Tripartite α-PFTs are members of the ClyA α-PFT family. Proteins in this family undergo a large scale conformational change from a compact soluble structure, where the hydrophobic residues are hidden often within a β-tongue motif, to an extended pore structure with the hydrophobic residues exposed in two extended α-helices which insert into the cell membrane. Here we show that S. marcescens has a tripartite haemolytic α-PFT (SmhABC), and propose a mechanism of pore assembly. We present the structures of the soluble A component (SmhA), as well as the soluble and pore conformations of the B component (SmhB).

To further investigate the differences in lytic activity between SmhABC and AhlABC the crystal structure of soluble SmhA was determined to 2.78 Å in space group P212121. This crystal form contained four closely related molecules in the asymmetric unit (rmsD Cα between molecules of 0.4–0.6 Å), with no oligomeric structures observed. SmhA folds into two distinct domains, a compact five helical bundle (α1, α2, α3, α6 and α7), and an associated head domain containing two helices (α4 and α5), and the β-tongue domain (two long anti-parallel β-strands, β1 and β2). In all monomers, there is missing density for approximately 20 residues between β1 and β2 (G208 – A229). Residues E192-V205 (β1 and loop to α3) and Y231-N250 (β2 and loop to α4) of the β-tongue domain are largely hydrophobic containing only polar uncharged and nonpolar residues, and are buried in the core of the protein, packing against α1, α3, α4, α5 (residues A272-Q283), and residues N351-E367 at the C-terminus. However, in SmhA, NheA and Hbl-B, this region has an additional extended loop and short helix that extends the length of the tail domain, a feature not observed in SmhB or AhlB. AhlB and SmhB use both a short β-strand and a short helix connected by a loop, while SmhA uses only a short loop perpendicular to β1. As soluble SmhA, SmhB and AhlB all share very similar structures, we propose that the head domain of SmhA would also unfold into its pore form about 2 hinges in the same way as seen in SmhB and AhlB, with hinge 1 between α3 and α4, and α5 and α6, and hinge 2 between α4 and β1, and α5 and β2. This would result in the pore form of SmhA having a similar extended helical structure to that of AhlB and SmhB. In this model the mixed hydrophobic/hydrophilic residues of the β-tongue head of SmhA form two extended amphipathic helices 36 Å in length at the ends of α3 and α4,, sufficient to cross the membrane, and thus with the potential to form a hydrophilic lining to the pore.

>[4x]MNNLTSIDLSPQTLMAMHISISSQALLNQSYSNLLLSQQLLTSQSMDPGLTVKIKAYQNQLRQQAQVFKQNTVAELIGLYTKASNFAALVNAVNALYSTEDPQVSQKGAEMVAALSDVAQHYQAAAQAVHTQLQAKREMLEPLMGNFLNVIDAIEQGLNAEAKQQAQTIAELNEAIAKNIQSIADAGFKAGEGVVQLGQSIVAAVPLGPTDKKPKEAPTAPPKPLSDQASYMISGIQAISAGASGAQQAVNELKANYAKLAVAYRALATANALLSVAKSVQAQAQLFVDTYVLTEQRMALLPTEWGKVAEAYLTAAPIINQAGSAAEIKQAKQIISLNAEKWQLFSKSIDNAKANYAGNNILPEVLEHHHHHH(3R,4S)-1-[(4-amino-5H-pyrrolo[3,2-d]pyrimidin-7-yl)methyl]-4-({[3-(1-butyl-1H-1,2,3-triazol-4-yl)propyl]sulfanyl}methyl)pyrrolidin-3-ol | C21 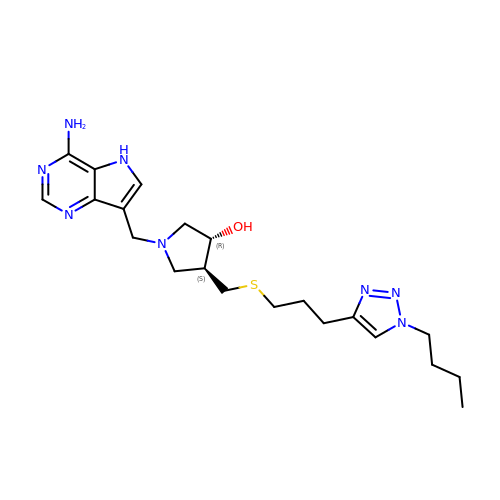H32 N8 O S | RDPUFRZNTDIFPO-AEFFLSMTSA-N>MENLNHCPLEDIKVNPWKTPQSTARVITLRVEDPNEINNLLSINEIDNPNYILQAIMLANAFQNALVPTSTDFGDALRFSMPKGLEIANTITPMGAVVSYVDQNVTQTNNQVSVMINKVLEVLKTVLGVALSGSVIDQLTAAVTNTFTNLNTQKNEAWIFWGKETANQTNYT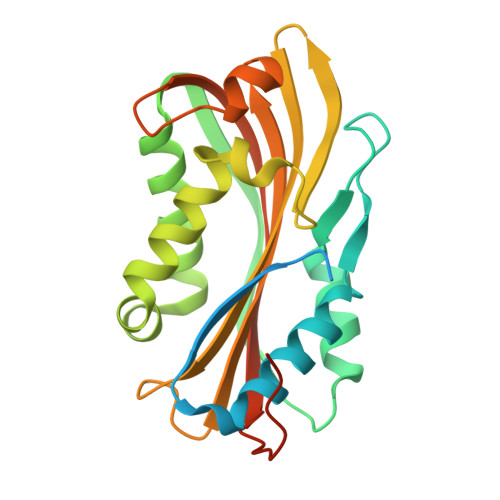YNVLFAIQNAQTGGVMYCVPVGFEIKVSAVKEQVLFFTIQDSASYNVNIQSLKFAQPLVSSSQYPIADLTSAINGTL[2x]ALLYL-{6-[3-(4-BROMO-PHENYL)-1-METHYL-1H-INDAZOL-6-YL]OXY}HEXYL)-N-METHYLAMINE | C24 H30 Br N3 O | 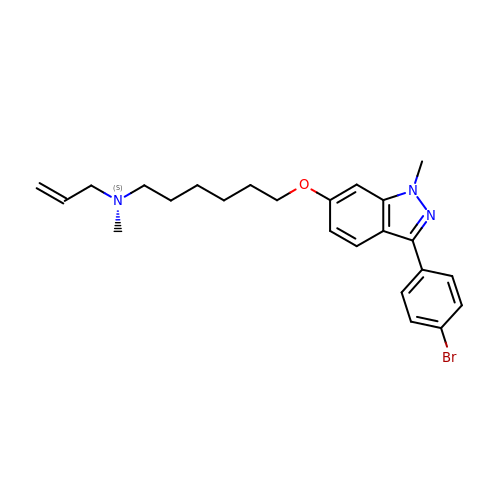FNZKIJOTNKEJBF-UHFFFAOYSA-N>[2x]GAMDRPGPPEGPVVISGVTAEKCTLAWKPPLQDGGSDIINYIVERRETSRLVWTVVDANVQTLSCKVTKLLEGNEYTFRIMAVNKYGVGEPLESEPVVAKNPFVVPDAPKAPEVTTVTKDSMIVVWERPASDGGSEILGYVLEKRDKEGIRWTRCHKRLIGELRLRVTGLIENHDYEFRVSAENAAGLSEPSPPSAYQKACDPIYKPGPPNNPKVIDITRSSVFLSWSKPIYDGGCEIQGYIVEKCDVSVGEWTMCTPPTGINKTNIEVEKLLEKHEYNFRICAINKAGVGEHADVPGPIIVEE

Titin is an intrasarcomeric protein filament of vertebrate striated muscle that plays essential roles in sarcomere development, passive mechanics and homeostatic regulation. Despite its large size, titin has a simple modular structure, primarily consisting of small immunoglobulin (Ig) and fibronectin type III (FnIII) domains (ca. 100 residues in length) that account for over 90% of its mass. Tandems composed of FnIII and Ig domains are found in titin’s A-band that is an integral component of the thick filament. The C(central)-zone extends along the myosin filament up to the edge of the bare zone and is formed by 11 copies of a long 11-domain tandem unit consisting of [Ig-(FnIII)2-Ig-(FnIII)3-Ig-(FnIII)3].

In order to obtain a domain structure representative of group B and to expand the understanding of FnIII domain arraying in titin’s A-band, we sought to elucidate the crystal structures of the triple FnIII-tandems A80-A82 and A84-A86 (both tandems of type ABC) from the C4 super-repeat, which PaSiMap analysis reveals to be a prototypical representative of titin’s C-zone. At the domain level, individual FnIII components were structurally equivalent in both molecular copies (RMSDCα values of 0.84 Å, 0.35 Å and 0.44 Å across copies of A84, A85 and A86 domains, respectively; calculated using UCSD Chimera, Pettersen et al. 2004). Regarding overall conformation, the crystal structure of A84-A86 reveals the poly-Fn tandem chain in an extended arrangement where sequential domains display alternating torsions along the chain path. Domain pairs A84-A85 and A85-A86 are joined by 3 residue long linkers that are largely hydrophobic in composition, having sequence NPF and DPI, respectively. Direct contacts between domains that could provide stability and rigidity to the tandem conformation are not observed, with steric hindrance between linker groups and neighbouring domains favouring extended arrangements. The copies differ primarily in the opening and rotation angle of the A85-A86 pair, which varies moderately between copies. An analysis of phi and psi dihedral torsion angles of linker residues showed that domain repositioning is singly caused by a small rotation around the psi main chain angle of the proline residue (DPI) in the linker sequence joining both domains. The [N/Y]PF sequence, with its bulky hydrophobic residue components, appears to allow only minor interdomain flexibility as revealed by a comparison of the two molecular copies of A84-A86 in this study.>RVSPFGGLKRLPAGLLLGHGPIRMVLAILAFLRFTAIKPSLGLINRWGSVGKKEAMEIIKKFKKDLAAMLRIINAR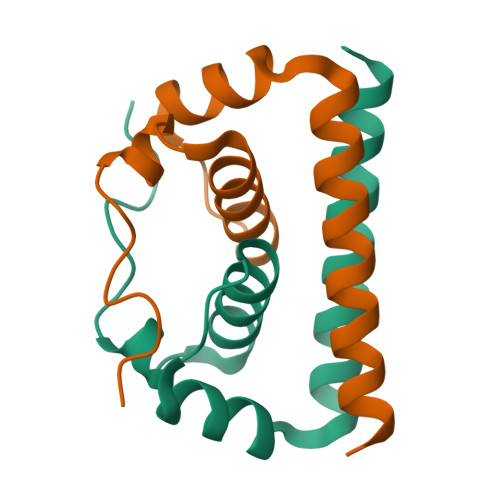[2x]> MTVTTTYPGVYLSEDAVSSFSVNSAATAVPLFAYDSENTNTINKPIQVFRNWAEFTVEYPTPLEDAFYTSLSLWFMHGGGKCYLVNEANIADAVAQYDDITLIVAAGTDTTTYTAFTTVVGQGYRIFGLFDGPKEKIAGTAKPDEVMEEYPTSPFGAVFYPWGTLASGAAVPPSAIAAASITQTDRTRGVWKAPANQAVNGVTPAFAVSDDFQGKYNQGKALNMIRTFSGQGTVVWGARTLEDSDNWRYIPVRRLFNAVERDIQKSLNKLVFEPNSQPTWQRVKAAVDSYLHSLWQQGALAGNTPADAWFVQVGKDLTMTQEEINQGKMIIKIGLAAVRPAEFIILQFSQDIAQ;> MATVTSVPGVYIEEDASPAMSVSASATAVPLFVARFTPLKPELAGVITRIGSWLDYTILFDSNVPSSARVTVSSTAVEPSPEFDALETASSKATTTYTYQIDDTEVVDPTASVALRLYFQNGGGPCYLYPLEKADDNGPLAALPDLIDEVGEITLLASPDPDETYRTAVYGALAASLDQHKGYFLLADSVNGDAPSAVGGSAQVAVYYPNVEVPHTRKLDDAEVAIDGYLDDEGKAVTTLAALRVVNTEFAGEIAQSLSGDLSAPLSLPPSALIAGVYGKTDGERGVWKAPANVVLNGVSDVSVRVTNEQQAELNPKGINVIRHFSDRGLVVWGSRTQKDDDDWRYIPVRRLFDAAERDIKKALQPMVFEPNSQLTWKRVQTAIDNYLYRLWQQGALAGNKAEEAYFVRVGKGITMTQDEINQGKM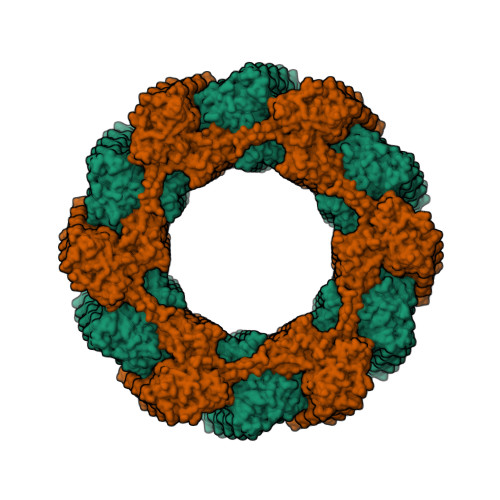IIQVGMAAVRPAEFIILKFTQDMSQ> GAQVSTQKTGAHETSLSATGNSIIHYTNINYYKDAASNSANR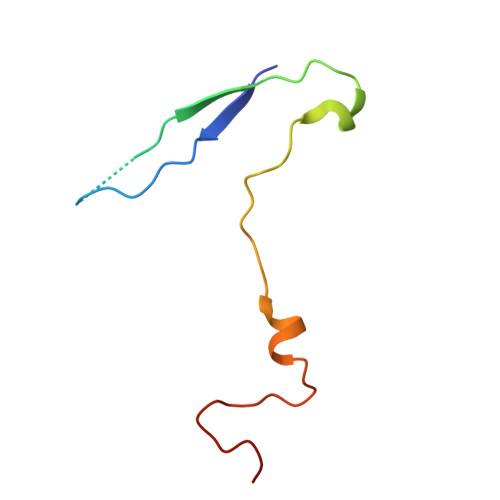QDFTQDPGKFTEPMKDVMIKTLPALN> MTMDEQQSQAVAPVYVGGFLARYDQSPDEARLLLPRDVVEHWLHAQGQGQPSLSVALPLNINHDDTAVVGHVAAMQSVRDGLFCLGCVTSPRFLEIVRRASEKSELVSRGPVSPLQPDK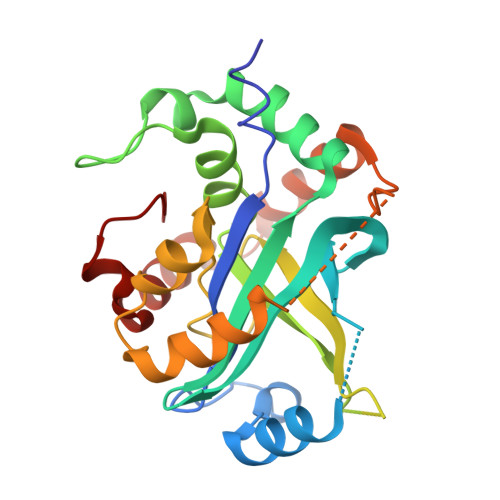VVEFLSGSYAGLSLSSRRCDDVEQATSLSGSETTPFKHVALCSVGRRRGTLAVYGRDPEWVTQRFPDLTAADRDGLRAQWQRCGSTAVDASGDPFRSDSYGLLGNSVDALYIRERLPKLRYDKQLVGVTERESYVKA>[2x]MNPQIRNPMKAMYPGTFYFQFKNLWEANDRNETWLCFTVEGIKRRSVVSWKTGVFRNQVDSETHCHAERCFL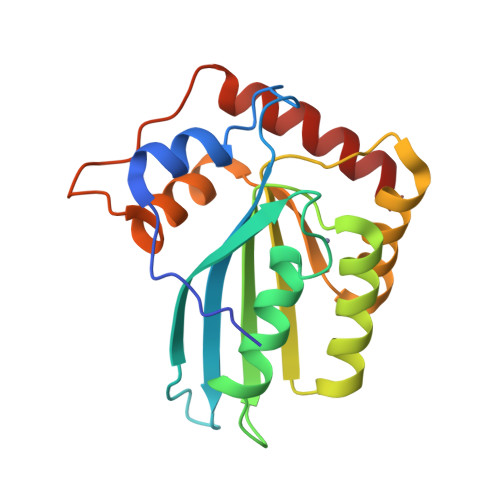SWFCDDILSPNTKYQVTWYTSWSPCPDCAGEVAEFLARHSNVNLTIFTARLYYFQYPCYQEGLRSLSQEGVAVEIMDYEDFKYCWENFVYNDNEPFKPWKGLKTNFRLLKRRLRESLQ methyl 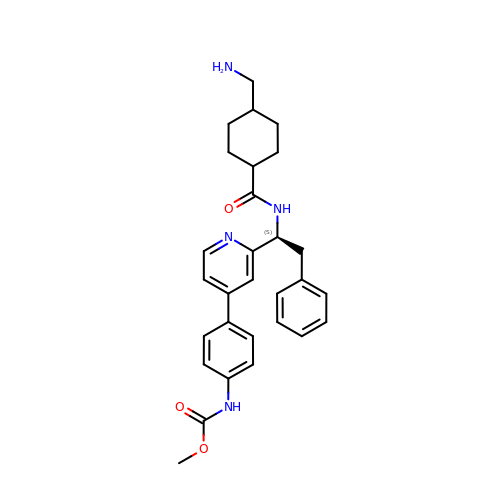~{N}-[4-[2-[(1~{S})-1-[[4-(aminomethyl)cyclohexyl]carbonylamino]-2-phenyl-ethyl]pyridin-4-yl]phenyl]carbamate | C29 H34 N4 O3 | YAJFVXIHHOXQOV-MYIHVTGJSA-N5-[(4-methylphenyl)sulfanyl]-1,2,3-thiadiazole-4-carboxylic acid | C10 H8 N2 O2 S2 | 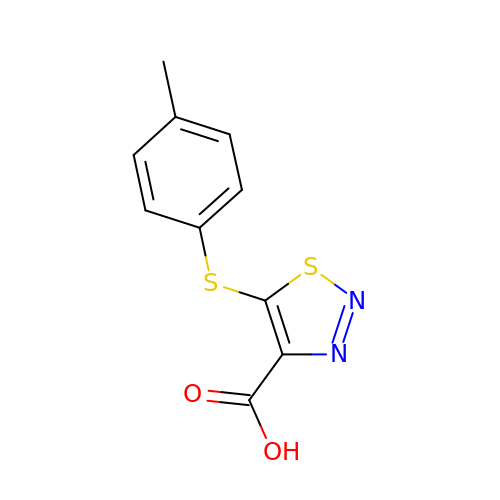PNOGJHWZHLJICV-UHFFFAOYSA-N(5Z,8Z,11Z,13S,14Z)-13-methylicosa-5,8,11,14-tetraenoic acid | C21 H34 O2 | 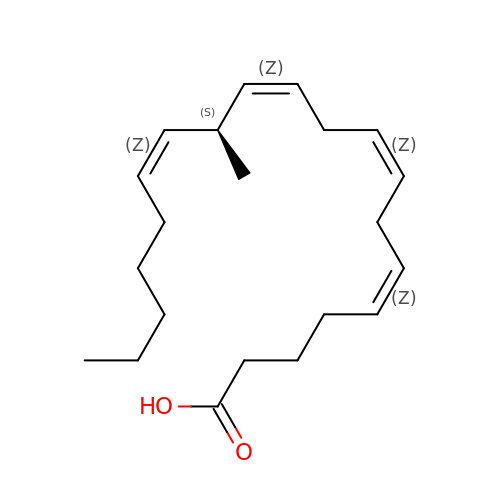PIZRMBAQQYSBSA-URRNNGNDSA-N>[8x]MNLKVKGARDVFEYMKGRIPDETKEHLFVLFLSTKNQILRHETITIGTLTASLIHPR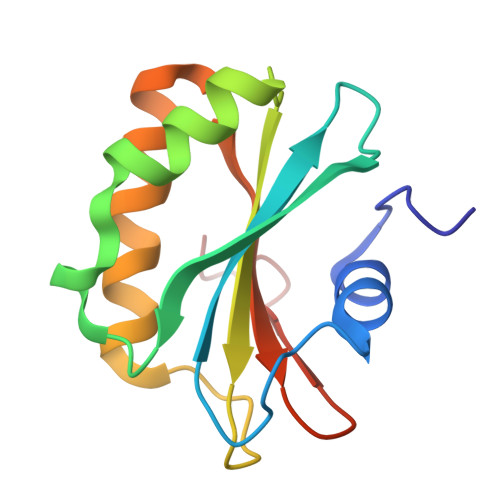EIFKAAIRESAHSIILVHNHPSGDVQPSNADKQVTSILKKAGDLLQIELLDHVIVGNNDWFSFRDHALL> GSKTISESELSASATELLQDYMLTLRTKLSSQEIQQFAALLHEYRNGASIHEFCINLRQLYGDSRKFLLLGLRPFIPEKDSQHFENFLETIGVKDGRG;> GSMDEQEALNSIMNDLVALQMNRRHRMPGYETMKNKDTGHSNRQSDVRIKFEHNGERRIIAFSRPVKYEDVEHKVTTVFGQPLDLHYMNNELSILLKNQDDLDKAIDILDRSSSMKSLRILLLSQD

MEKK3 (MAP3K3) is a highly conserved protein kinase essential for embryonic angiogenesis in mice. MEKK3 interacts physically with CCM2 but how this interaction is mediated, and its relevance to cerebral vasculature, are not known. MEKK3 contains only two defined domains: an N-terminal Phox/Bem1p (PB1) domain and a C-terminal catalytic domain. We find a direct interaction between the harmonin homology domain (HHD) of CCM2 and the N-terminal region of MEKK3 encompassing both an N-terminal helix and the Phox/Bem1p (PB1) domain, and determine a 2.35-Å cocrystal structure of the complex.

To better understand how CCM2 and MEKK3 interact we determined a cocrystal structure of MEKK3NPB1 with CCM2HHD to 2.35 Å resolution. In addition to the HHD and PB1 domains, we observed a stretch of positive difference density between CCM2HHD helices H1 and H2. This difference density corresponded to an additional helix, which, after further rounds of refinement, we identified and built as the N-terminal 19 residues of MEKK3. The overall structure of the CCM2HHD:MEKK3NPB1 complex reveals an extensive interface between the two proteins. MEKK3 resembles a hand, with the N-terminal helix forming the thumb and the PB1 domain forming the palm/fingers. MEKK3 grasps the CCM2HHD, with the thumb (MEKK3N) resting in the groove between CCM2 helices H1 and H2, and the palm/fingers (MEKK3PB1) holding CCM2 helices H2 and H3. The N-terminal helix (αN) of MEKK3 fits snugly into the hydrophobic groove between CCM2 helices H1/H4 and H2, making extensive interactions with them. We found that mutants in MEKK3 helix αN (A6D/L7D, D13R, I10D/L14D) severely interrupted CCM2 pull down, but mutation within the MEKK3 PB1 domain (L119E/L121E) only moderately reduced CCM2HHD pull down. Isothermal titration calorimetry showed an observed Kd of 1.4±0.4 μM for the wild-type (WT) components, but no heat of interaction was observed for CCM2HHD (A319D/A320D), MEKK3NPB1 (A6D/L7D) or MEKK3NPB1 (D13R) mutants tested. We therefore conclude that the interaction between CCM2 and MEKK3 is important for correct subcellular localization of CCM2.>[2x]MDSISLRVALNDGNFIPVLGFGTTVPEKVAKDEVIKATKIAIDNGFRHFDSAYLYEVEEEVGQAIRSKIEDGTVKREDIFYTSKLWSTFHRPELVRTCLEKTLKSTQLDYVDLYIIHFPMALQPGDIFFPRDEHGKLLFETVDICDTWEAMEKCKDAGLAKSIGVSNFNCRQLERILNKPGLKYKPVCNQVECHLYLNQSK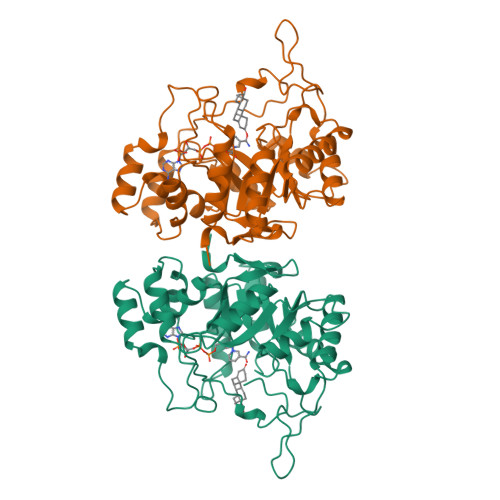MLDYCKSKDIILVSYCTLGSSRDKTWVDQKSPVLLDDPVLCAIAKKYKQTPALVALRYQLQRGVVPLIRSFNAKRIKELTQVFEFQLASEDMKALDGLNRNFRYNNAKYFDDHPNHPFTDEN> MQSSTSTDQHVLHHMDPHRFTSQIPTATSSQLRRRNSTNQGL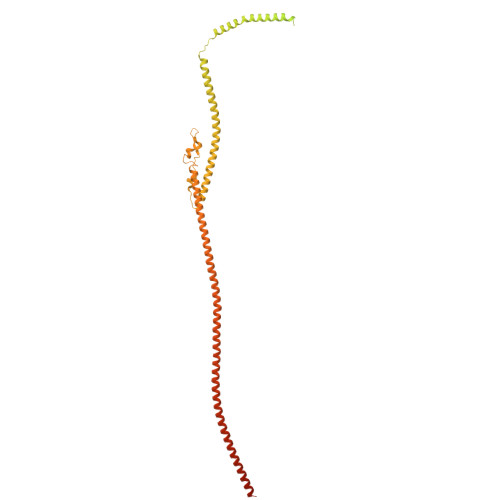TDMINKSIARNTISGTGIPTGGINKNKRTRSTVAGGTNGTALALNDKSNSRNSVSRLSINQLGSLQQHLSNRDPRPLRDKNFQSAIQEEIYDYLKKNKFDIETNHPISIKFLKQPTQKGFIIIFKWLYLRLDPGYGFTKSIENEIYQILKNLRYPFLESINKSQISAVGGSNWHKFLGMLHWMVRTNIKLDMCLNKVDRSLINQNTQEITILSQPLKTLDEQDQRQERYELMVEKLLIDYFTESYKSFLKLEDNYEPSMQELKLGFEKFVHIINTDIANLQTQNDNLYEKYQEVMKISQKIKTTREKWKALKSDSNKYENYVNAMKQKSQEWPGKLEKMKSECELKEEEIKALQSNISELHKILRKKGISTEQFELQNQEREKLTRELDKINIQSDKLTSSIKSRKLEAEGIFKSLLDTLRQYDSSIQNLTRSRSQLGHNVNDSSLKINISENLLDRDFHEGISYEQLFPKGSGINESIKKSILKLNDEIQERIKTIEKDNITLEKDIKNLKHDINEKTQINEKLELELSEANSKFELSKQENERLLVAQRIEIEKMEKKINDSNLLMKTKISDAEELVTSTELKLEELKVDLNRKRYKLHQQVIHVIDITSKFKINIQSSLENSENELGNVIEELRNLEFETEHNVTN Clostridium thermocellum has extensive potential in lignocellulose biorefineries as an environmentally prominent, thermophilic, cellulolytic bacterium. Previously, five putative sugar transporters, denoted A to D and L and belonging to the ABC transport systems group, were identified in the genome of C. thermocellum, and the solute-binding lipoproteins (SBP) of these ABC transporters were shown to bind different dextrins by isothermal titration calorimetry (ITC) assays. To gain insight into the structural mechanism of the transporter specificities, 11 crystal structures, both alone and in complex with appropriate saccharides, were solved for all 5 putative sugar-binding proteins, thus providing detailed specific interactions between the proteins and the corresponding saccharides. Combined genetic, biophysical, and structural studies have provided solid evidence that transporter A and transporter B are the major glucose and cellodextrin transporters, respectively, among the five potential sugar transporters in C. thermocellum.

Similar to the typical SBP fold, all of the Cbps adopted two-domain structures connected by three hinge regions, with the buried ligand-binding site between the two domains. The unliganded CbpB structure and the complex structures of CbpB with cellodextrins (G2 to G5) were determined to 1.70 to 2.00 Å resolution. A hinge motion was observed between the unliganded CbpB and its complexed structures, and the rigid body rotation angle was ~17°. CbpB showed high affinities for all of the tested cellodextrins (G2 to G5), with the highest affinity for cellotetraose (KD = 0.562 μM). Surprisingly, the growth phenotypes of these mutants indicated that transporter B is the sole cellodextrin transporter, whereas transporter A is the sole glucose transporter.

>SVKLTMWIMPNSDTPDQDLLKVVKPFTDANPHITVEPTVVDWSAALTKITAAATSGEAPDITQVGSTWTAAIGAMEGALVELTGKIDTSAFVESTLQSAYIKGTDKMFGMPWFTETRALFYRKDACEKAGVNPETDFATWDKFKDALKKLNGIEVDGKKLAALGMPGKNDWNVVHNFSWWIYGAGGDFVNEEGTQATFSSENALKGIKFYSELAVEGLMDEPSLEKNTSDIESAFGDGAYATAFMGPWVISSYTKNKEENGNDLIDKIGVTMVPEGPAGRYAFMGGSNLVIFNSSKNKDEALELLKFFASKEAQVEYSKVSKMLPVVKAAYEDPYFEDSLMKVFKEQVDKYGKHYASVPGWASAEVIFSEGLSKIWDNVMEVDGAYSYDKTVQIVKDVESQINQILQETSK[2x]>MTEPLPRIQHYEDLGLGLFIHWGLYSQMAVGEWTELIHHRNQHDYEQLIKTFTAAQFDAKKIAHAAKAVGAKYIVLTTKHHEGFFLYDTKGLSDFDVMHAPARRDLIAEFVAACREEDLLPFFYMATYDWHTPLYDDDFPAYLTYLQKSVEVLCRNYGPVGGFWFDGNWNKKDADWHLPELYGMIRHYQPNAIIVNNTGLKNRGQVSDPEIDVVTYERRTPDEIYHGAPNEKYVAGEISITLNQHWGIAANDLNYKSPAEVIETVAHARHIGANILVNIGLTGTG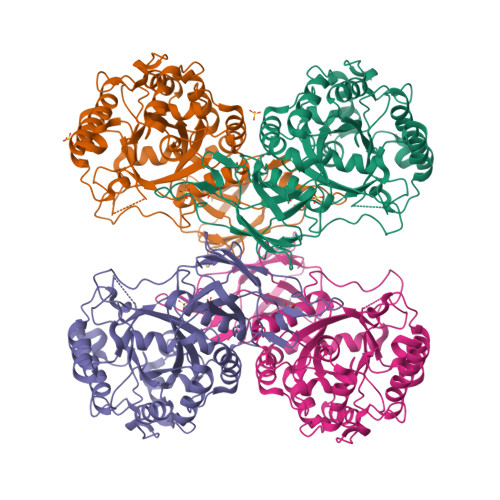AIPAAAQTYMHLLGRWTAMAAPVLYKGRPVPVTSAHGTRDFVLHTSKHDFLCILDLQVVGNDNVVLGGEGVNPRSFVGIGQPIQRIHWLDNDEVLSFTQDLDKKVLTVDATGYPYGSDWVVRIAQIDYE[8x]> MALEEIRPKEVYLDRKLLTLEDKELGSG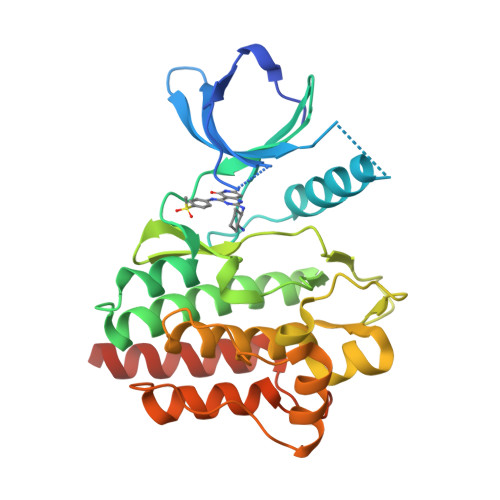NFGTVKKGYYQMKKVVKTVAVKILKNEANDPALKDELLAEANVMQQLDNPYIVRMIGICEAESWMLVMEMAELGPLNKYLQQNRHVKDKNIIELVHQVSMGMKYLEESNFVHRDLAARNVLLVTQHYAKISDFGLSKALRADENYYKAQTHGKWPVKWYAPECINYYKFSSKSDVWSFGVLMWEAFSYGQKPYRGMKGSEVTAMLEKGERMGCPAGCPREMYDLMNLCWTYDVENRPGFAAVELRLRNYYYDVVNLEHHHHHHHH>GTGDGSMSTPAPAFDRD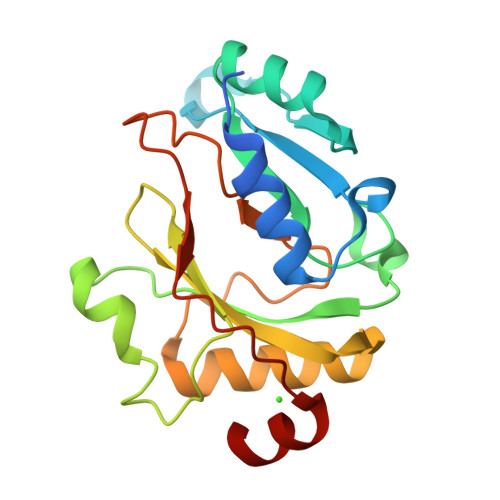QILLHLSLLRKDIATTRYRAIWPRREDKVKAWTTPLTGATVQDAVTQGFNSYIVVGDGGDSDAEITSVNAIFGEWDDGDLAWQVGAWEACGLPRPSFQLRTGGKSIHHYWVFHSPVDVPAWTELQARLIALAGFDTTNRNPSRVMRLAGCPHQRTGEVAQIFNATGELYDPGQMLQVLP[2x]> SEVIEGNVKIDRISPGDGATFPK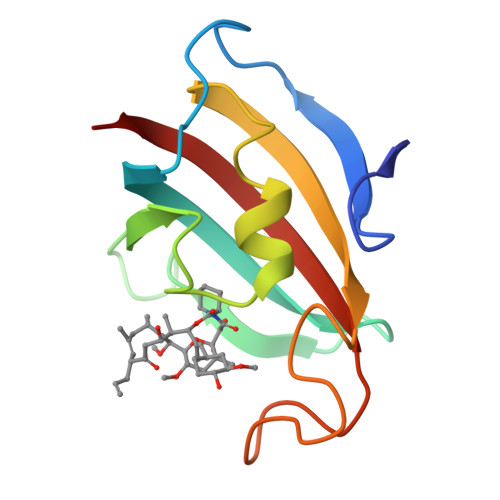TGDLVTIHYTGTLENGQKFDSSVDRGSPFQCNIGVGQVIKGWDVGIPKLSVGEKARLTIPGPYAYGPRGFPGLIPPNSTLVFDVELLKVN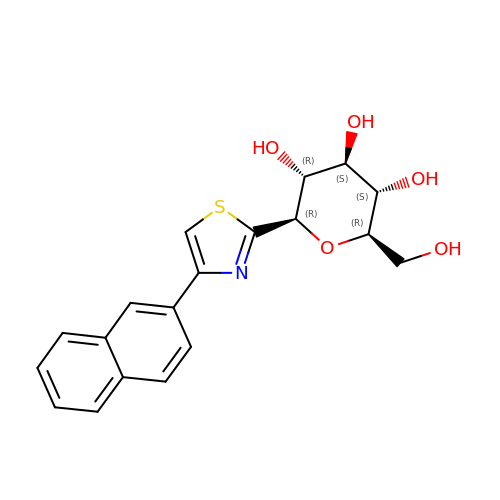(2~{R},3~{S},4~{S},5~{R},6~{R})-2-(hydroxymethyl)-6-(4-naphthalen-2-yl-1,3-thiazol-2-yl)oxane-3,4,5-triol | C19 H19 N O5 S | NRPWZWOXDUROHO-UYTYNIKBSA-N> METVAYADFARLEMRVGKIVEVKRHENADK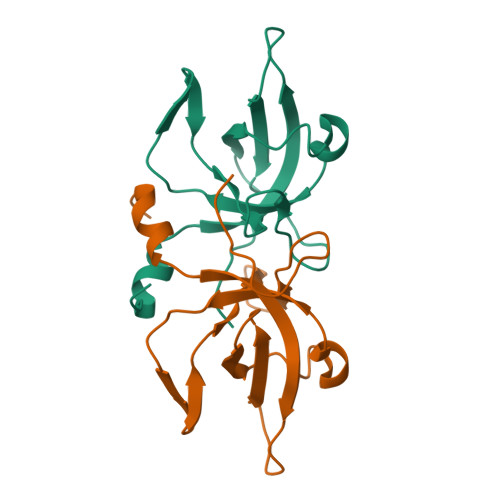LYIVQVDVGQKTLQTVTSLVPYYSEEELMGKTVVVLCNLQKAKMRGETSECMLLCAETDDGSESVLLTPERMMPAGVRVVLDHHHHHH>[2x]GTSLKQAYAQGFLLGTAVNADIVSGKDAASAALVACHFNAVTAENVMKAEVVAPRRGVQDFSAADAFVAYAQRDRQFVVGHTLVWHNQTPEWFFTTADGRPNTPAQQLERMRAHIAAVAGRYTGKVQAWDVVNEIIDEDGSYRSTNWVQRVGDGDTVVRNAFAFAQRYAPDAQLYYNDFNAWRPAKREGIVRMVKMLQQAGVRIDGVGMQGHWGLNYPSLRDIEDAIDAYAALGVKVMITELDIDVLP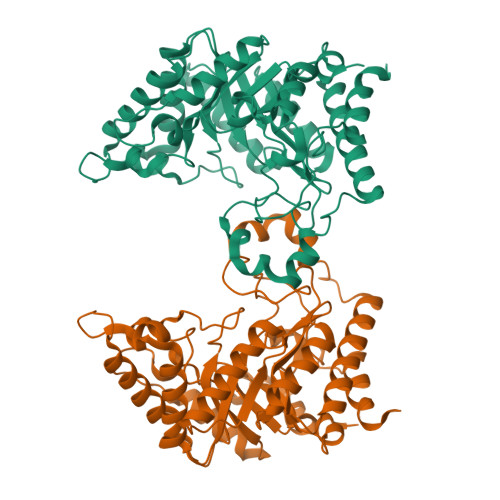LTKEGQIIGTGMAHKQFQLPEFKRFLDPYRDGLPADVQAQLRDRYAELFALFWRKRDKIARVSVWGVSDDMSWKNDYPVPGRTNYPLLFDRNHQPKPALDAVVAVPSAT>[2x]ASASEQETLVRPKPLLLKLLK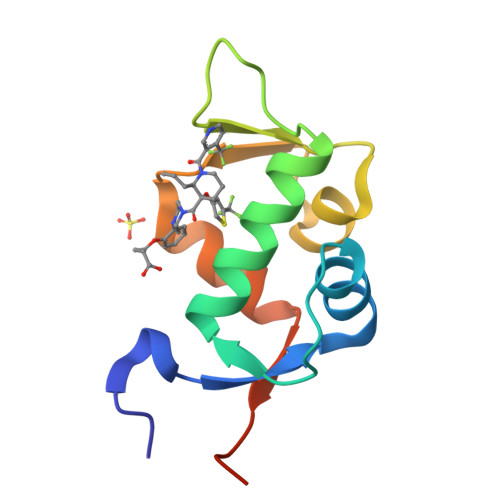SVGAQKDTYTMKEVLYYLGQYIMTKRLYDEKQQHIVHCSNDLLGDLFGVPSFSVKEHRKIYTMIYRNLVVVNQQESSAGA>[4x]SMLAELITSYRKSIAIYTFVDTGLSVHFKNGTYMDINELASQYGIDYSRLNRLCDFLIEIGVLVSSNDRVALSEECRVLADPESMESLIAKWEFNSGLWNAWLMYPKSLLENNGKSAFEIANGKPFFEYL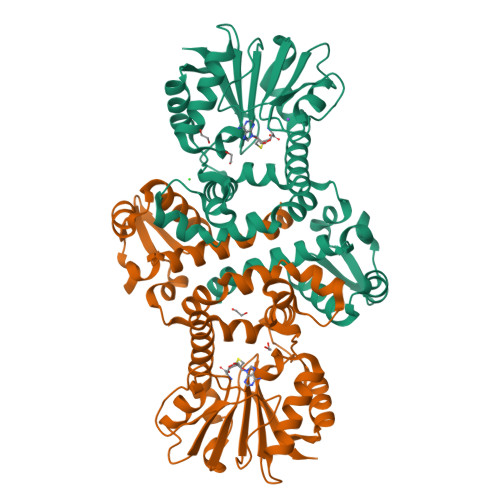DSNKLLKSKFDSLMSKDSDKMIEKLFNVYDFNQHDKILDVGGGEGNLLIRMSEKVKEKHYAVLDRYNELPDYGNINFIDGDFFKSIPSGYDLYILKNVIHDWPDNDAILILENCRKAMGNNATILLITLMKKPQSNIIKYFDILMDVSSLGKERDLTEFEYLANQAGLVIQDVKDIDESYSIIQLGVK>MAHHHHHHMSAAPRIGILGAGGRMGRILIQAVQQAGYQLGAAVVRPESTLIGADAGELAGIGSIGVKLTGSLAEVLEDCDVVIDFSTPAATSEHLKLCREAGVAIVIGTTGMSDEQKAELDETAKHIPVVYAANYSVGVNVSIKLLELAAKVFGDTVDIEVIEAHHRHKVDAPSGTALMMGEAIADTLGRNLKEVAVYGREGHTGPRDRQTIGFETIRGGDIVGEHTVMFIGEGERVEVTHKATNRMNFAAGAVRAAA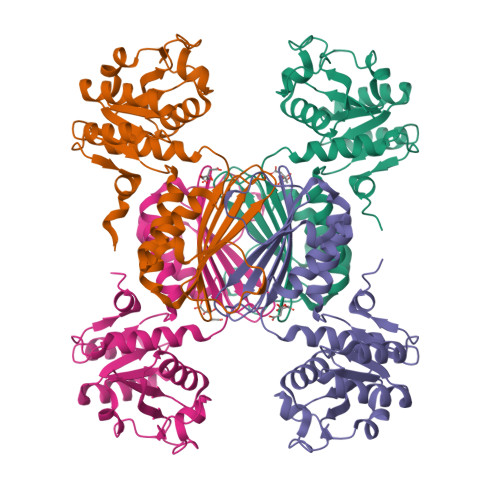WVVGREARKYDMKDVLGLNDVQV[6x]> NPCLTGPRTCKDLLDRGHFLSGWHTIYLPDCRPLTVLCDMDTDGGGWTVFQRRVDGSVDFYRDWATYKQGFGSRLGEFWLGNDNIHALTAQGTSELRTDLVDFEDNYQFAKYRSFRVADEAEKYNLVLGAFVEGSAGDSLTFHNNQSFSTKDQDNDLNTG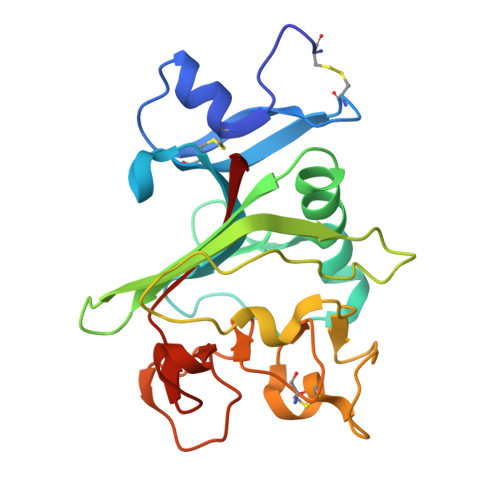NCAVMFQGAWWYKNCHTSNLNGRYLRGTHGSFANGINWKSGKGYNYSYKVSEMKVRPA>[3x]IIEFHVIGNSLTPKANRRVLLWLVGLQNVFS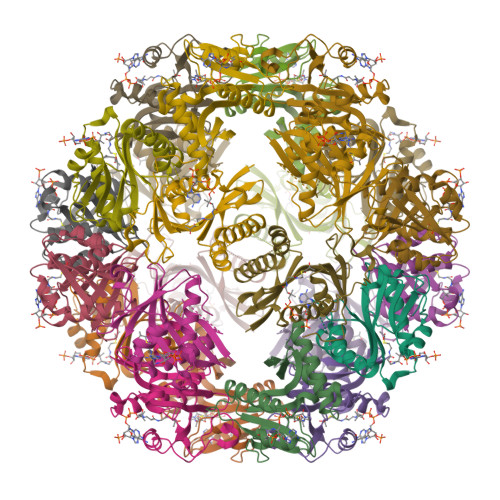HQLPRMPKEYIARLVFDPKHKTLALIKDGRVIGGICFRMFPTQGFTEIVFCAVTSNEQVKGYGTHLMNHLKEYHIKHNILYFLTYADEYAIGYFKKQGFSKDIKVPKSRYLGYIKDYEGATLMECELNPRIPYT>[2x]MRID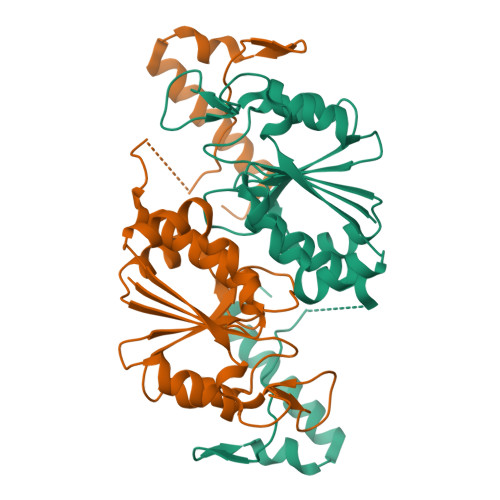IVTIFPACLDPLRQSLPGKAIESGLVDLNVHDLRRWTHDVHHSVDDAPYGGGPGMVMKAPVWGEALDEICSSETLLIVPTPAGVLFTQATAQRWTTESHLVFACGRYEGIDQRVVQDAARRMRVEEVSIGDYVLPGGESAAVVMVEAVLRLLAGVLGNPASHQDDSHSTGLDGLLEGPSYTRPASWRGLDVPEVLLSGDHARIAAWRREVSLQRTRERRPDLSHPDGSHHHHHH> QDLDYKDDDDKMSGTKLEDSPPCRDWSSASELDETQEPLLDPTDYDDEEFLRYLWREYLHPKEYAWVLIAGYIIVFVVALIGNVLVCVAVWKNHHMRTVTNLFIVNLSLAAVLVTITCLPATLVVDITETWFFGQSLCKVIPYLQTVSVSVSALTLSCIALDRWYAICHPLMFKSTAKRALNSIVIIWIVSCIIMIPQAIVMECSTVFPGLADKTTAFTVCDERWGGEI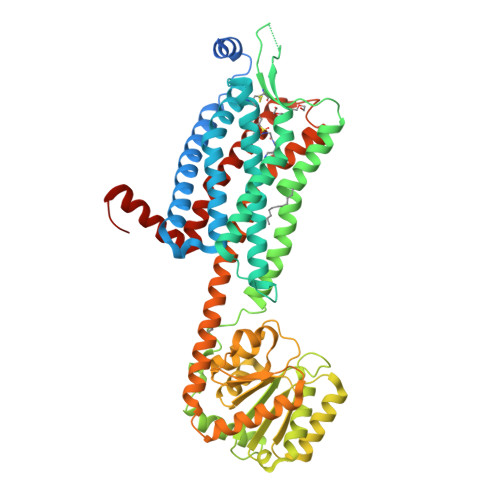APKMYHICFFLVTYAAPLCLMVLLYLQIFRKLWCRQGIDCSFWNESYLTGSRDERKKSLLSKFGMDEGVTFMFIGRFDRGQKGVDVLLKAIEILSSKKEFQEMRFIIIGKGDPELEGWARSLEEKHGNVKVITEMLSREFVRELYGSVDFVIIPSYFEPFGLVALEAMCLGAIPIASAVGGLRDIITNETGILVKAGDPGELANAILKALELSRSDLSKFRENCKKRAMSFSKQIRARRKTARMLMVVVLVFAICYAPISILNVLKRVFGMFAHTEDRETVYAWFAFSHWLVYANSAANPIIYNFLSGKFREEFKAAFSWWWLGVHHHHHHHHHH1,3-diazinan-2-one | C4 H8 N2 O | 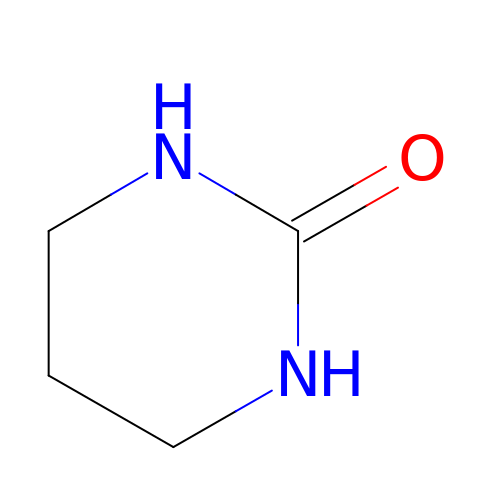NQPJDJVGBDHCAD-UHFFFAOYSA-N> MKKEKNDPTTPGTTTTVIPLQTTVQTPITLGSANNFAVIAGSSVTNTGATNITGDLGLSPGTSIGGFPPGILNGTLHINDAIANQAKLDITTAYNDAAARVASDMVTISGNIGGLTLTPGLYKSTSSLAVSSGDVTFDALGDPSAIFVIQIASTLTTTPGRKVLLSGGALASNIYWQVSSSASFGTTTSFKGTVIALESITFD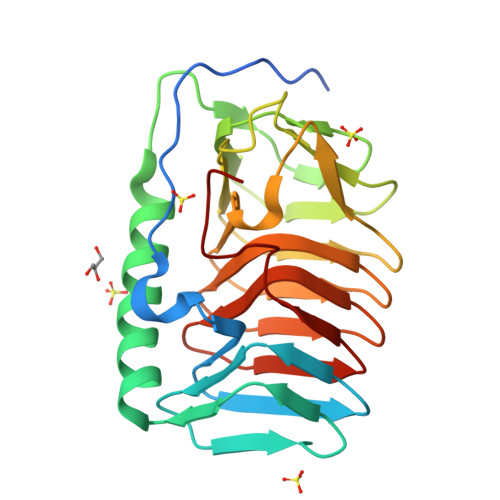TGATLEGRALARNGAVTMEGNTFVLPLEHHHHHH> DKATIPSESPFAAAEVADGAIVVDIAKMKYETPELHVKVGDTVTWINREAMPHNVHFVAGVLGEAALKGPMMKKEQAYSLTFTEAGTYDYHCTPHPFMRGKVVVE;> APQFFNIIDGSPLNFDDAMEEGRDTEAVKHFLETGENVYNEDPEILPEAEELYAGMCSGCHGHYAEGKIGPGLNDAYWTYPGNETDVGLFSTLYGGATGQMGPMWGSLTLDEMLRTMAWVRHLYTGDPKDASWLTDEQKAGFTPFQP;> QGQAAARAAAADLAAGQDDEPRILEAPAPDARRVYVNDPAHFAAVTQQFVIDGEAGRVIGMIDGGFLPNPVVADDGSFIAHASTVFSRIARGERTDYVEVFDPVTLLPTADIELPDAPRFLVGTYPWMTSLTPDGKTLLFYQFSPAPAVGVVDLEGKAFKRMLDVPDCYHIFPTAPDTFFMHCRDGSLAKVAFGTEGTPEITHTEVFHPEDEFLINHPAYSQKAGRLVWPTYTGKIHQIDLSSGDAKFLPAVEALTEAERA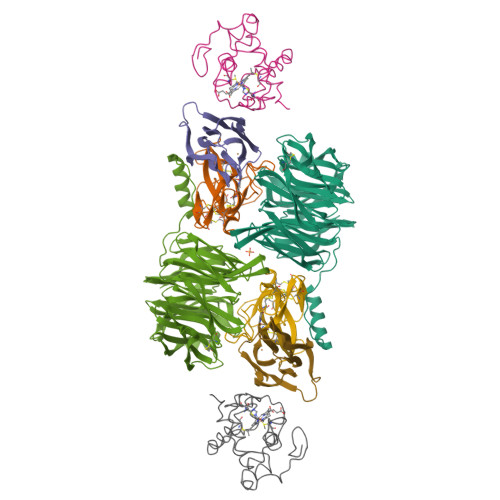DGWRPGGWQQVAYHRALDRIYLLVDQRDEWRHKTASRFLVVLDAKTGERLAKFEMGHEIDSINVSQDEKPLLYALSTGDKTLYIHDAESGEELRSVNQLGHGPQVITTADMG;> TDPRAKWVPQDNDIQACDYWRHCSIDGNICDCSGGSLTNCPPGTKLATASWVASCYNPTDGQSYLIAYRDCCGYNVSGRCPCLNTEGELPVYRPEFANDIIWCFGAEDDAMTYHCTISPIVGKAS Virulent phages belonging to the newly created Skunavirus genus (previously 936) are by far the most predominant in dairy factories and they currently belong to the Siphoviridae family (double-stranded DNA genome and non-contractile tail) of the Caudovirales order. Phage p2 is the model phage for this viral genus and it infects L. lactis MG1363, a laboratory strain used in many studies on Gram-positive bacteria. Of interest here, phage p2 uses a multi-protein baseplate at the tip of its tail to bind to its cell wall polysaccharide (CWPS) receptor at the host cell surface. Here, we present further structural analyzes of the phage p2 baseplate, proposing a topological model of the baseplate resting state, and interpreting a new nsEM structure of the virion, in its active conformation.

However, when Ca2+ (or Sr2+) was added to the purified baseplate complex, the baseplate exhibited a different conformation in which the receptor-binding domains point downwards in the direction opposite to the capsid. In addition, the Tal trimer adopted an open conformation instead of a closed one in the purified baseplate-VHH5 complex. In both baseplate conformations, an extension of the Dit galectin domain, the “arm”, holds the RBPs by inserting its “hand” within the trimeric RBP “shoulder” domain. In this context, it was proposed that the structure obtained in the presence of Ca2+ was an actived form of the phage baseplate. It was also suggested that the baseplate transition from resting to activated state could be the trigger for Tal opening and subsequent release of the tail tape measure protein (TMP), followed by DNA ejection. However, we were unable to obtain this baseplate activated state in p2 virions, despite many attempts, which included the addition of divalent cations (Ca2+, Sr2+), hampering somewhat the validity of the suggested activation mechanism.

>MLEANVYDNFNPNYYNISDFSMPNGKKEKRGLPIPKARCQVINYELWETGYLYTSSATLTVSVEVGDIVQILFPEVVPIEEALGKKKKLNLDMVYLVTDVDESNKATLKNYFWAMIESLDVPNAITKTTNFAIIDYLIDPNKNNLMSYGYFFNSSIFAGKATINRKAETSSAHDVAKRIFSKVQFQPTTTIQHAPSETDPRNLLFINFASRNWNRKRITTRVDIKQSVTMDTETIVERSAYNFAVVFVKNKATDDYTDPPKMYIAKNNGDVIDYSTYHGDGTDLPDVRTAKTLFYDRDDHGNPPELSTIKVEISPSTIVTRLIFNQNELLPLYVNDLVDIWYEGKLYSGYIADRVKTEFNDRLIFVESGDKPNVI[3x];>[12x]MVRQYKIHTNLDGTDDKVWDVTNGKVRFYQPSNLGLQSTNNIWQSNGIGVMGTRSITQPQIEFKLETFGESLEENYQLMKDFVNDILSKKFVTLEYQTEIFQVYADLALADVTKTEGYGKNGTFSEKITFDIITKWYTYENLTFDKIQNGKVIAGMSKIYGGTAPGNYKYIKGTSYTYYGESDIDRLSRWDIKEEIFSFMGILYPKLPKTPAGVRFLDDIGNEYTAIVFKTEQVQDYILINTDVNDETYQGWKGTTALNLFPVMDFERYRTRIIEKGQMELINLSKAEFKIKRKADFV;>MTIKNFTFFSPNSTEFPVGSNNDGKLYMMLTGMDYRTIRRKDWSSPLNTALNVQYTNTSIIAGGRYFELLNETVALKGDSVNYIHANIDLTQTANPVSLSAETANNSNGVDINNGSGVLKVCFDIVTTSGTGVTSTKPIVQTSTLDSISVNDMTVSGSIDVPVQTLTVEAGNGLQLQLTKKNNDLVIVRFFGSVSNIQKGWNMSGTWVDRPFRPAAVQSLVGHFAGRDTSFHIDINPNGSITWWGANIDKTPIATRGNGSYFIK[18x]> AKLGAVYTEGGFVEGVNKKLGLLGDSVDIFKGIPFAAPTKALENPQPHPGWQGTLKAKNFKKRCLQATITQDSTYGDEDCLYLNIWVPQGRKQVSRDLPVMIWIYGGAFLMGSGHGANFLNNYLYDGEEIATRGNVIVVTFNYRVGPLGFLSTGDANLPGNYGLRDQHMAIAWVKRNIAAFGGDPDNITLFGESAGGASVSLQTLSPYNKGLIRRAISQSGVALSPWVIQKNPLFWAKKVAEKVGCPVGDAARMAQCLKVTDPRALTLAYKVPLAGLEYPMLHYVGFVPVIDGDFIPDDPINLYANAADIDYIAGTNNMDGHIFASIDMPAINKGNKKVTEEDFYKLVSEFTITKGLRGAKTTFDVYTESWAQDPSQENKKKTVVDFETDVLFLVPTEIALAQHRANAKSAKTYAYLFSHPSRMPVYPKWVGADH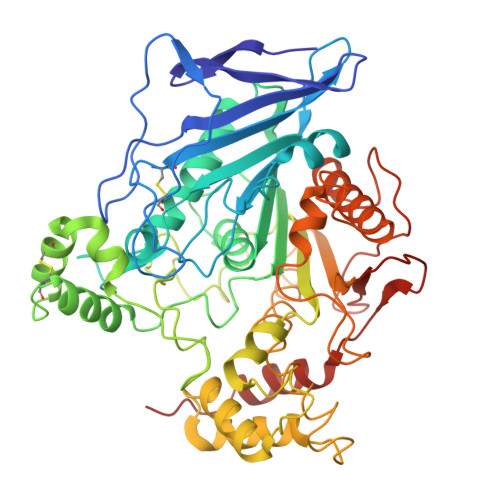ADDIQYVFGKPFATPTGYRPQDRTVSKAMIAYWTNFAKTGDPNMGDSAVPTHWEPYTTENSGYLEITKKMGSSSMKRSLRTNFLRYWTLTYLALPTVT> MKTVVFAYHDMGCL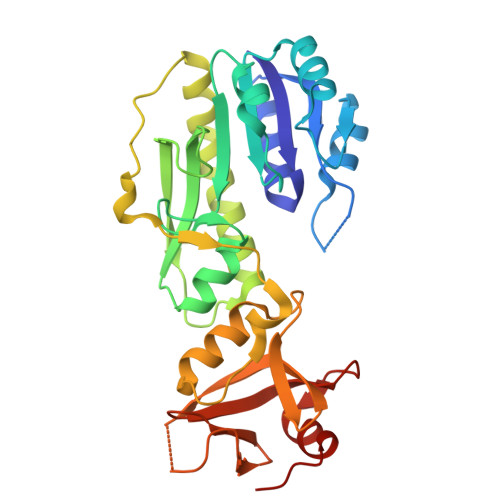GIEALLAAGYEISAIFTHTDNPGEKAFYGSVARLAAERGIPVYAPDNVNHPLWVERIAQLSPDVIFSFYYRHLIYDEILQLAPAGAFNLHGSLLPKYRGRAPLNWVLVNGETETGVTLHRMVKRADAGAIVAQLRIAIAPDDIAITLHHKLCHAARQLLEQTLPAIKHGNILEIAQRENEATCFGRRTPDDSFLEWHKPASVLHNMVRAVADPWPGAFSYVGNQKFTVWSSRVHPHASKAQPGSVISVAPLLIACGDGALEIVTGQAGDGITMQGSQLAQTLGLVQPG> GHMKIKIVPAVGGGSPLELEVAPNATVGAVRTKVCAMKKLPPDTTRLTYKGRALKDTETLESLGVADGDKFVLITRTVGG

The first complete archaeal Ub modifier system, including E2 and E3 enzymes, was discovered in 2011 in Candidatus Caldiarchaeum subterraneum. C. subterraneum Ub (CsUb), E1, E2, and E3 are organized in a single operon, adjacent to a second E3 protein and a JAMM protease (CsRpn11) with high sequence similarity to eukaryotic Rpn119. We have shown that CsRpn11 is highly active on its own, cleaving both CsUb precursors and, at a later stage of the ubiquitination cascade, CsUb-conjugated substrate proteins. Our bioinformatic, structural, and biochemical results reveal unique features of the archaeal proteins, but also remarkable conceptual similarities with their eukaryotic counterparts.

Fitting to the thermophilic nature of C. subterraneum, CsUb is an extremely thermostable monomeric protein (Tm > 95 °C in circular dichroism heat-denaturation studies). The CsUb gene encodes for a precursor of 87 amino acids (Ub-pre). We could solve the structure via molecular replacement using human ubiquitin as a search model, revealing for CsUb the classical β-grasp fold with a two-residue insertion in the first-loop region. Likewise, a cluster analysis of Ub-like proteins reveals eukaryote-like Ub sequences in E2- and E3-containing archaea, while other prokaryotes only encode for more distant homologs. Again, the closest connections to eukaryotic ubiquitin are made by sequences from Asgard archaea and Caldiarchaeum (dark violet, magenta; enlarged inset), CsUb being up close with 31% sequence identity.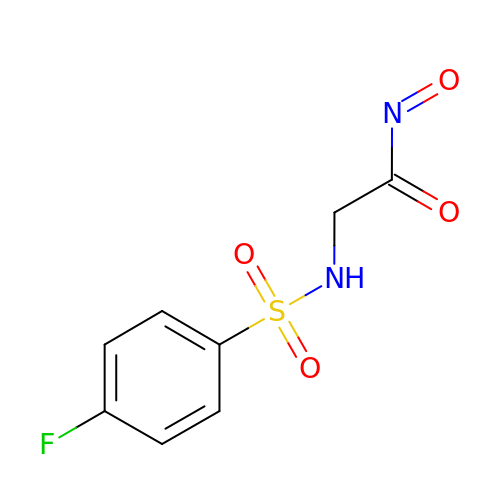2-[(4-fluorophenyl)sulfonylamino]-N-oxo-ethanamide | C8 H7 F N2 O4 S | ATANXIMWDMRRIO-UHFFFAOYSA-N The abnormal expansion of GGGGCC/GGCCCC hexanucleotide repeats (HR) in C9orf72 is associated with amyotrophic lateral sclerosis (ALS) and frontotemporal dementia (FTD). On the RNA level, bidirectional transcription produces sense and antisense transcripts containing complementary regions of repeated stretches of GGGGCC (G4C2) and GGCCCC (G2C4) that form stable secondary and tertiary structures. Overall, the RNA folded into a parallel triplex-like motif flanked by double-stranded duplexes and terminated by single-stranded cytosines. The triplex motif was composed of four C+•G-C pairs representing standard major groove base triples (C+ denotes protonated cytosine).

In the unliganded structure, the cytosines formed a peculiar triplex i-motif, assembled by trans C•C+ pair and a third cytosine located at the Hoogsteen edge of the C•C+ pair. The two terminal cytosines of chain A, which were bound to ANP77 in the liganded structure, engaged in higher-order interactions. They formed peculiar C•C+•C base triples assembled by symmetry-related residues (5C of chain A, 6C of symmetry-related chain A, and 6C of symmetry-related chain D). The base triples consisted of a trans C•C+ pair commonly found in i-motif structures. The C•C+ pair formed three hydrogen bonds via Watson–Crick edges. The third C from the triples was located in the Hoogsteen edge of one of the cytosine residues from the i-motif pair. The unique triplex-i-motif observed in ligand-free G2C4 RNA has not yet been described. In the unliganded structure two magnesium cations were observed. Both of them directly interacted with oxygen atoms of the phosphate groups of RNA. For the phosphate groups, being in close proximity, their high negative charge was usually neutralized by Mg2+ ions as it was observed in unliganded structure.

>[4x]GGCCCC5-METHYLPYRIDIN-2-AMINE | C6 H8 N2 | 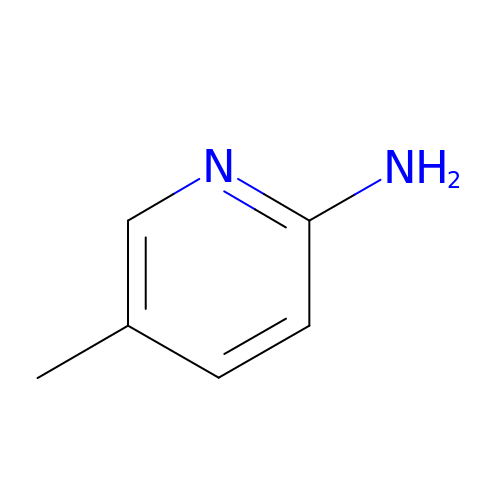CMBSSVKZOPZBKW-UHFFFAOYSA-N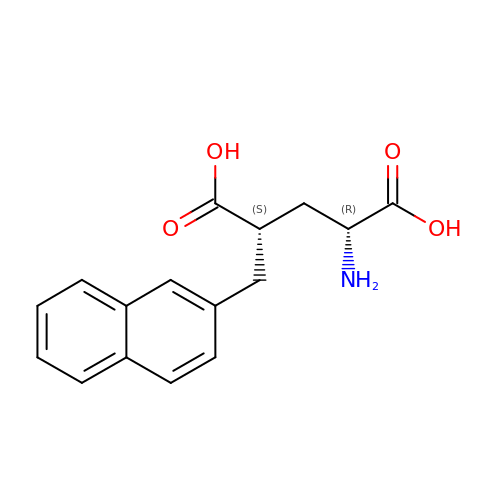(4S)-4-(2-NAPHTHYLMETHYL)-D-GLUTAMIC ACID | C16 H17 N O4 | YDWIUFASTTZKNI-UONOGXRCSA-N>[2x]APLHIDTALPDAAQIQQSNSWLEISLGQFQSNIEQFKSHMNANTKICAIMKADAYGNGIR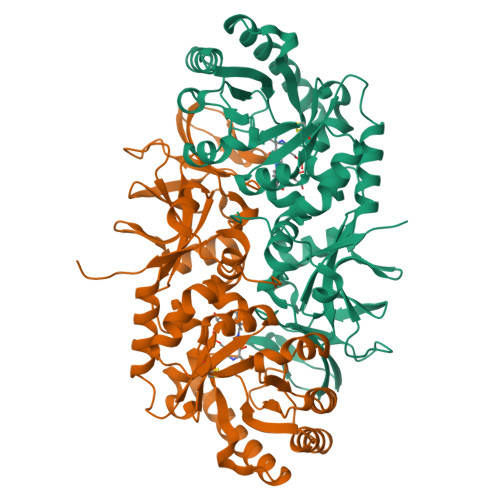GLMPTIIAQGIPCVGVASNAEARAVRESGFKGELIRVRSASLSEMSSALDLNIEELIGTHQQALDLAELAKQSGKTLKVHIALNDGGMGRNGIDMTTEAGKKEAVSIATQPSLSVVGIMTHFPNYNADEVRAKLAQFKESSTWLMQQANLKREEITLHVANSYTALNVPEAQLDMVRPGGVLFGDLPTNPEYPSIVSFKTRVSSLHHLPKDSTVGYDSTFTTSRDSVLANLPVGYSDGYPRKMGNKAEVLINGQRAKVVGVTSMNTTVVDVTEIKGVLPGQEVVLFGQQQKQSIAVSEMENNAELIFPELYTLWGTSNPRFYVKENLYFQ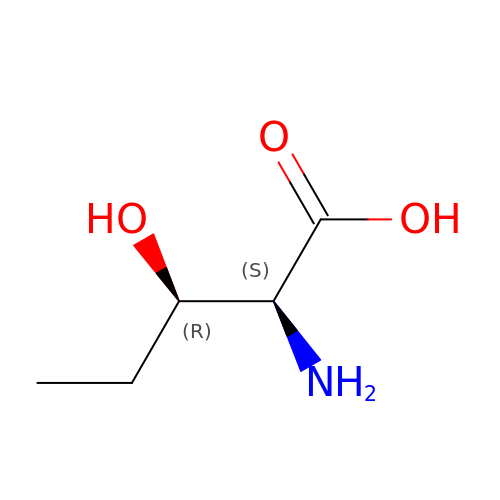(3R)-3-hydroxy-L-norvaline | C5 H11 N O3 | LGVJIYCMHMKTPB-DMTCNVIQSA-N>MITVRKIKLTIMGDKDTRNSQYKWIRDEQYNQYRALNMGMTYLAVNDILYMNESGLEIRTIKDLKDCEKDIDKNKKEIEKLTARLEKEQNKKNSSSEKLDEIKYKISLVENKIEDYKLKIVELNKILEETQKERMDIQKEFKEKYVDDLYQVLDKIPFKHLDNKSLVTQRIKADIKSDKSNGLLKGERSIRNYKRNFPLMTRGRDLKFKYDDNDDIEIKWMEGIKFKVILGNRIKNSLELRHTLHKVIEGKYKICDSSLQFDKNNNLILNLTLDIPIDIVNKKVSGRVVGVDLGLKIPAYCALNDVEYIKKSIGRIDDFLKVRTQMQSRRRRLQIAIQSAKGGKGRVNKLQALERFAEKEKNFAKTYNHFLSSNIVKFAVSNQAEQINMELLSLKETQNKSILRNWSYYQLQTMIEYKAQREGIKVKYIDPYHTSQTCSKCGNYEEGQRESQADFICKKCGYKVNADYNAARNIAMSNKYITKKEE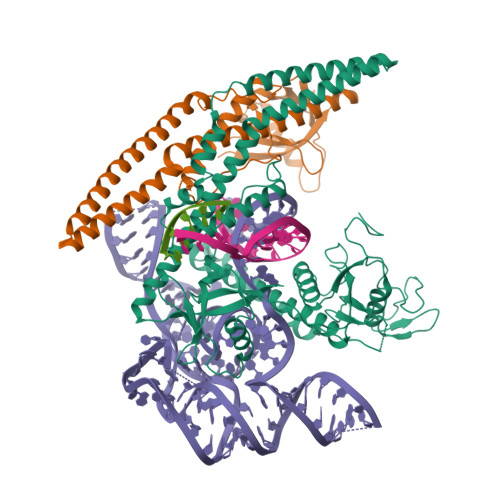SKYYKIKESMV[2x]>MSARRTESDIQGFHATPEFGGNLQKVLVDLIELSLQGKQAHWNVVGSNFRDLHLQLDELVDFAREGSDTIAEEMRALDAVPDGRSDTVAATTTLPEFPAFERSTADVVDLITTRINATVDTIRRVHDAVDAEDPSTADLLH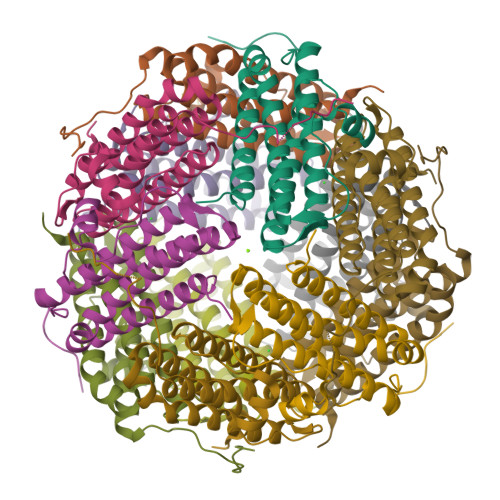GLIDGLEKQAWLIRSENRKV[4x]> SKKRQWALEDFEIGRPLGKGKFGNVYLAREKQSKFILALKVLFKAQLEKAGVEHQLRREVEIQSHLRHPNILRLYGYFHDATRVYLILEYAPLGTVYRELQKLSKFDEQRTATYITELANALSYCHSKRVIHRDIKPENLLLGSAGELKIADF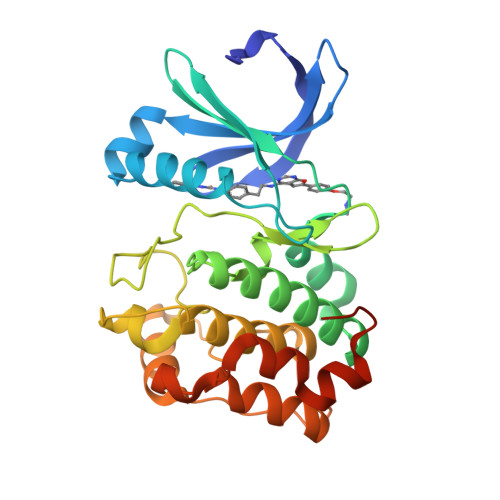GWSVHAPSSRRTDLCGTLDYLPPEMIEGRMHDEKVDLWSLGVLCYEFLVGKPPFEANTYQETYKRISRVEFTFPDFVTEGARDLISRLLKHNPSQRPMLREVLEHPWITANSSKPSNCQNKESASK>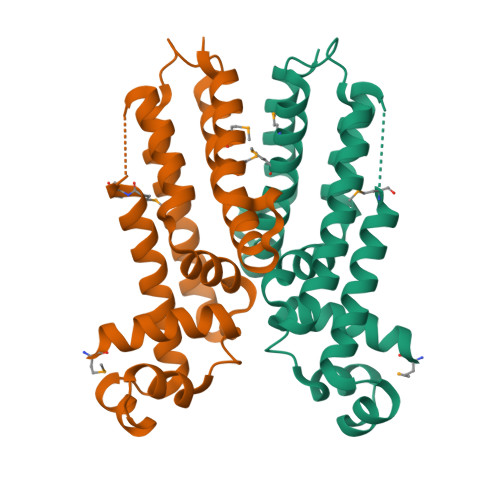[2x]MHHHHHHMKDKIIDNAITLFSEKGYDGTTLDDISKSVNIKKASLYYHYDNKEEIYRKSVENCFNYFIDFMMRNHDDNYSIDGLYQFLFKFIFDVDERYIKLYVQLSSAPEALNSEIKHHLQEINTTLHDELIKYYDPTHIALDKEDFINMILMFLETWYFRASFSQKFGIIEDSKNRFKDQVYSLLNVFLKK> MNEGRIFLYVSP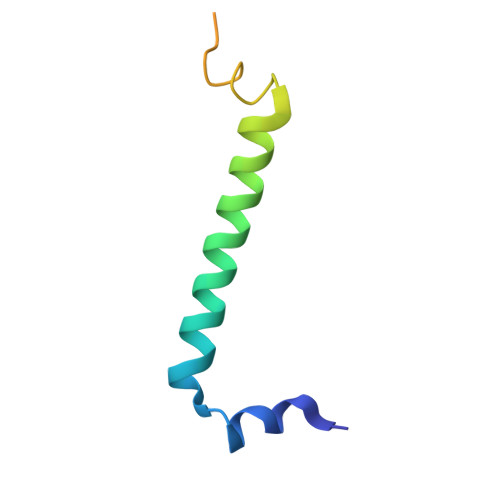EVILPIMFLILVLTSLTVHFAILINTTWFGDFFQGSAGEFAAAPAAADANAAPWE One such Rab15 effector is Rep15, which is known to have a role in receptor recycling from the endocytic recycling compartment but otherwise remains poorly characterized. Biochemical validation of the interactions is presented and crystal structures of the Rep15:Rab3B and Rep15:Rab3C complexes provide additional mechanistic insight. We find that Rep15 adopts a globular structure that is distinct from other reported Rab15, Rab3 and Rab34 effectors. Detailed biochemical studies reveal that Rep15 is selective for Rab15, Rab3 paralogs and Rab34 and does not bind to other evolutionarily similar Rab GTPases.

To do this, we either mixed purified Rep15 and Rabs at 1:1 ratio or co-expressed and purified Rep15 ΔN1:Rab3AQ81L_19-217, Rep15 ΔN1:Rab3BQ81L_18-190 and Rep15 ΔN1:Rab34Q111L_1-237 complexes. All obtained complexes were used to perform the crystallization screen and finally, we obtained crystals for Rep15:Rab3CGppNHp_Q222H_10-227 (bovine), Rep15:Rab3BGppNHp and Rep15_ΔN1:Rab3BQ81L_18-190 complexes. Subsequently, we also obtained Rep15:Rab3BGppNHp and Rep15 ΔN1:Rab3BQ81L_18-190 complex crystals, which diffracted to a resolution 2.75 Å and 2.8 Å, respectively and crystallized in space group C2 and P21 respectively. We solved the Rep15:Rab3B complex structure using Rep15:Rab3C (bovine) as a MR model and Rep15 ΔN1:Rab3BQ81L_18-190 complex structure using Rep15:Rab3BGppNHp complex structure as a MR model. The asymmetric unit contained two copies of the complex. Both copies share nearly the same overall architecture, as indicated by an RMSD of 0.124 Å for Rep15:Rab3BGppNHp complex and and an RMSD of 0.109 Å for the both copies of Rep15 ΔN1:Rab3BQ81L_18-190 complex. Structurally-based sequence alignment of Rab3A and Rab3C shows that apart from the switch I, interswitch and switch II residues, three RabCDRs of Rab3A are involved in making contacts with the Rabphilin-3A, whereas in the case of the Rep15:Rab3 complex structures, RabCDRs are not part of the binding interface.

>[2x]GHMVPVVCEVVSEAIVHAAQKLKEYLGFEYPPSKLCPAANTLNEIFLIHFITFCQEKGVDEWLTTTKMTKHQAFLFGADWIWTFWGSDKQIKLQLAVQTLQMSSPPPVESKPCDLSNPESRVEESSWKKSRFDKLEEFCNLIGEDCLGLFIIFGMPGKPKDIRGVVLDSVKSQMVRSHLPGGKAVAQFVLETEDCVFIKELLRNCLSKKDGLREVGKVYISIL;>MNFDYMFKLLIIGNSSVGKTSFLFRYADDTFTPAFVSTVGIDFKVKTVYRHEKRVKLQIWDTAGLERYRTITTAYYRGAMGFILMYDITNEESFNAVQDWATQIKTYSWDNAQVILVGNKCDMEEERVVPTEKGQLLAEQLGFDFFEASAKENISVRQAFERLVDAICDKMSDS[2x]> MADNLPSDFDVIVIGTGLPESIIAAACSRSGQRVLHVDSRSYYGGNWASFSFSGLLSWLKEYQENNDVVTENSMWQEQILENEEAIPLSSKDKTIQHVEVFCYASQDLHKDVEEAGALQKNHASVTSAQSAEAAEAAETSCLPTAVEPLSMGSCEIPAEQSQCPGPESSPEVNDAEATGKKENSDAKSSTEEPSENVPKVQDNTETPKKNRITYSQIIKEGRRFNIDLVSKLLYSRGLLIDLLIKSNVSRYAEFKNITRILAFREGTVEQVPCSRADVFNSKQLTMVEKRMLMKFLTFCVEYEEHPDEYRAYEGTTFSEYLKTQKLTPNLQYFVLHSIAMTSETTSCTVDGLKATKKFLQCLGRYGNTPFLFPLYGQGELPQCFCRMCAVFGGIYCLRHSVQCLVVDKESRKCKAVIDQFGQRIISKHFIIEDSYLSENTCSRVQYRQISRAVLITDGSVLRTDADQQVSILTVPAEEPGSFAVRVIELCSSTMTCMKGTYLVHLTCMSSKTAREDLERVVQKLFTPYTEIEAENEQVEKPRLLWALYFNMRDSSDISRDCYNDLPSNVYVCSGPDSGLGNDNAVKQAETLFQQICPNEDFCPAPPNPEDIVLDGDSSQQEVPESSVTPETNSETPKESTVLGNPEE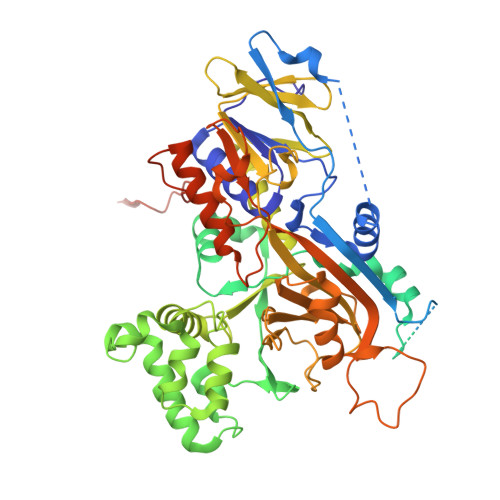PSE{[(7-carbamimidoylnaphthalen-2-yl)methyl][4-({1-[(1E)-ethanimidoyl]piperidin-4-yl}oxy)phenyl]sulfamoyl}acetic 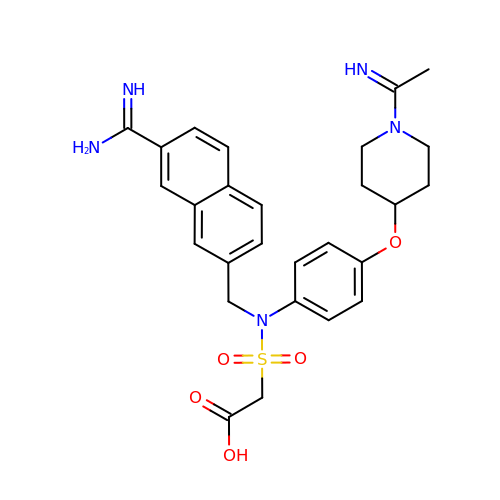acid | C27 H31 N5 O5 S | NPBKHEMDWREFJJ-MTDXEUNCSA-N> MNVYFLGGGNMAAAVAGGLVKQGGYRIYIANRGAEKRERLEKELGVETSATLPELHSDDVLILAVKPQDMEAACKNIRTNGALVLSVAAGLSVGTLSRYLGGTRRIVRVMPNTPGKIGLGVSGMYAEAEVSETDRRIADRIMKSVGLTVWLDDEEKMHGITGISGSGPAYVFYLLDALQNAAIRQGFDMAEARALSLATFKGAVALAEQTGEDFE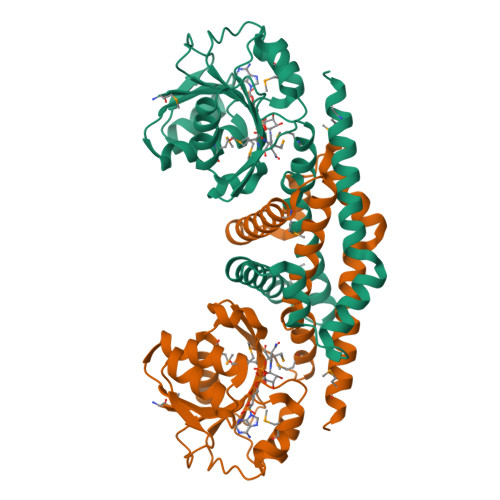KLQKNVTSKGGTTHEAVEAFRRHRVAEAISEGVCACVRRSQEMERQYQ>MHHHHHHSIKQNCLIKIINIPQGTLKAEVVLAVRHLGYEFYCDYIDGQAMIR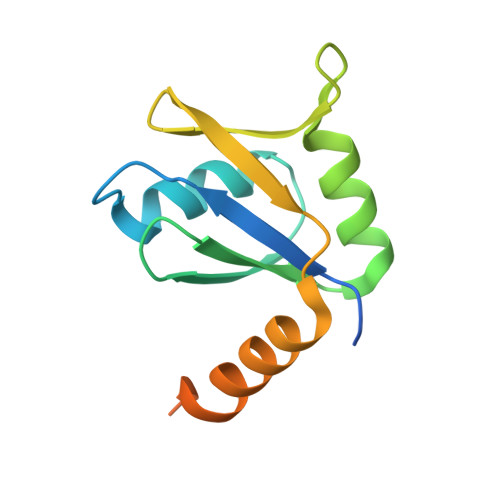FQNSDEQRLAIQKLLNHNNNKLQIEIRGQICDVISTIPEDEEKNYWNYIKFKKNEFRKFFFMKKQQKKQNITQNYNK[6x]>GMAYAQWVIIIIHNVGSQDVKIKNLKASWGKLHADGDKDAEVSASNYEGKIVKPDEKLQINASGRSDAAEGTTGTFDLVDPADGDKQVRHFYWDSPWGSKTNTWTVSGSNTKWMIEYSGQNLDSGALGT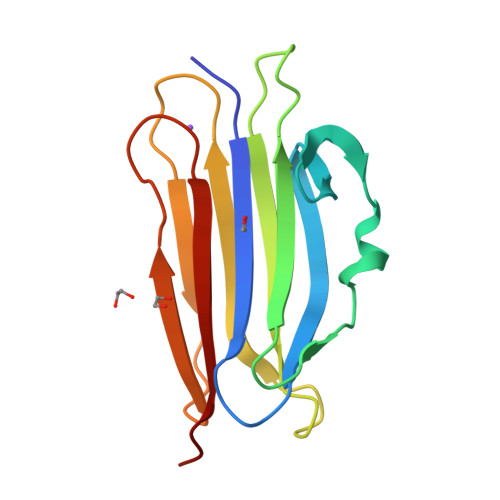ITVDTLKKGN[4x]>[22x]MDADKIVFKVNNQVVSLKPEIIVDQHEYKYPAIKDLKKPCITLGKAPDLNKAYKSVLSGMSAAKLDPDDVCSYLAAAMQFFEGTCPEDWTSYGIVIARKGDKITPGSLVEIKRTDVEGNWALTGGMELTRDPTVPEHASLVGLLLSLYRLSKISGQNTGNYKTNIADRIEQIFETAPFVKIVEHHTLMTTHKMCANWSTIPNFRFLAGTYDMFFSRIEHLYSAIRVGTVVTAYEDCSGLVSFTGFIKQINLTAREAILYFFHKNFEEEIRRMFEPGQETAVPHSYFIHFRSLGLSGKSPYSSNAVGHVFNLIHFVGCYMGQVRSLNATVIAACAPHEMSVLGGYLGEEFFGKGTFERRFFRDEKELQEYEAAELTKTDVALADDGTVNSDDEDYFSGETRSPEAVYTRIMMNGGRLKRSHIRRYVSVSSNHQARPNSFAEFLNKTYSSDS

As for all non-segmented negative RNA viruses, rabies virus has its genome packaged in a linear assembly of nucleoprotein (N), named nucleocapsid. RABV N is composed of two globular domains that are connected by a hinge, creating an RNA binding groove. It also comprises two subdomains, an N-terminal extension, named the NNT-ARM, and an internal loop in the C-terminal domain, named the NCT-ARM, that dock to neighboring subunits in the polymeric form and thereby stabilize the assembled NC. Thus, genome replication requires the production of the unassembled RNA-free N protein, named N0, in the form a complex named the N0−P complex, in which P prevents the polymerization of N and the illegitimate assembly with cellular RNA until N is transferred to nascent viral RNA.

The structural alignments using PDBeFold showed that NCTD in our refined NΔ230−P68 structure was similar to that in the N−RNA complex (RMSD = 0.84 Å), while the NNTD exhibited some differences with residues from 35 to 103 and from 189 to 200 being out-of-register in the structural alignment despite an RMSD of 0.95 Å. An analysis of the original electron density map of the N−RNA complex revealed that the absence of density for residues from 105 to 118 and 185 to 188 and the low resolution of density had resulted in the incorrect positioning of the latter region relative the remaining NNTD (see below). For NΔ230−P68, the C-terminal part of P68 (res from 42 to 68 + tag) remained flexible and sampled a wide range of conformations, consistent with the SAXS-based ensemble analysis. In the MD simulations of the N3−RNA system, the C-terminal domains remained stable as previously found, but the N-terminal domains started to unfold in the first 100 ns of the simulation, reflecting possible packing defects due to the incorrect construction of the protein segment from residue from 135 to 200 (see above). We thus re-refined the N11−RNA model against the original dataset using more recent software and the model of N extracted from the NΔ230−P68 structure (built from higher resolution data), which yielded an improved model of the circular undecameric N−RNA complex. Using three adjacent N subunits (N3−RNA) from the re-refined N−RNA complex structure, the MD simulations showed that the N protein structure was stable over several hundred ns in multiple independent trajectories. The first crystal structures of polymeric, circular N−RNA complexes revealed that the RNA molecule was embedded in its protein shell, with some bases facing the protein away from the solvent. This directly suggested that the N protein must open and close, with the NNTD and NCTD moving relative to each other by rotation around a hinge located in their connecting region. The binding of RNA, NNT-ARM, and also NCT-ARM blocks N in a close conformation that shields the RNA from the solvent, cellular proteins, and the viral polymerase.> ADYKVYPWGLNDPTEGSRVMIKDPWDTVASEFTWNSDGTKKYPTTRGNNGIAQSNPSGEDDYINNHRPRSSNLSFNYPYSPSSSPPSSYIDASIVQLFYTANMYHDLLYTLGFTEKTGNFEFNNNGQGGRGNDYVILNSQDGSGTNNANFATPPDGQPGRMRMYTWTKSQPYRDGSFEAGIVIHEYTHGVSNRLTGGPANSNCLSTIEAGGMGEGWGDFMATAIRLKAADTRAKDYTMGAWAANDPKGIREYPYSTSLTTNPLAYSNVDGDDSVHSIGTVWATMLYELMWNLIDKHGKNVSAKPTMKGGVPTDGKYLAMKLVVDGMALQPCNPNFVQA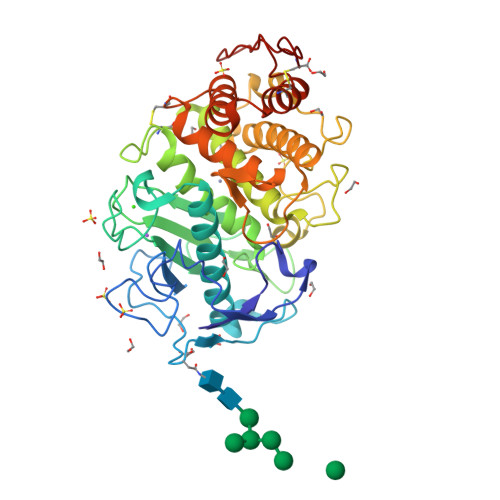RDAILDADKALTKGANRCEIWKAFAKRGLGYGAKYNENKRVTSNKLPSGC> MKELIYIEEPKILFAHGQKCTDARDGLALFGPLNNLYGIKSGVIGTKQGLKIFRDYLDHIQKPIYNSNSITRPMFPGFEAVFDCKWESTGITFKEVTNEDIGKFLYNSSTHKRTYDLVSLFIDKIISANKNEDENVDVWFVIVPDEIYKYCRPNSVLPKEMVQTKALMSKSKAKSFRYEPSLFPDINIELKEQEKEAETYNYDAQFHDQFKARLLKHTIPTQIFRESTLAWRDFKNAFGLPIRDFSKIEGHLAWTISTAAFYKAGGKPWKLSDVRNGVCYLGLVYKKVEK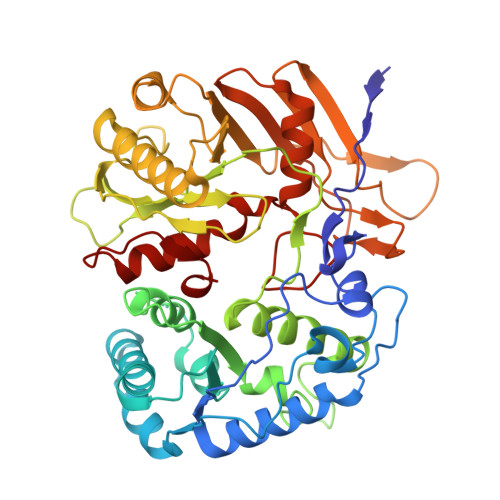SKNPRNACCAAQMFLDNGDGTVFKGEVGPWYNPKNGQYHLEPKEAKALLSQSLQSYKEQIGEYPKEVFIHAKTRFNHQEWDAFLEVTPKETNLVGVTISKTKPLKLYKTEGDYTILRGNAYVVNERSAFLWTVGYVPKIQTALSMEVPNPLFIEINKGEADIKQVLKDILSLTKLNYNACIFADGEPVTLRFADKIGEILTASTDIKTPPLAFKYYI>[4x]MPPMLSGLLARLVKLLLGRHGSALHWRAAGAATVLLVIVLLAGSYLACLAERGAPGAQLITYPRALWWSVETATTVGYGDLYPVTLWGRL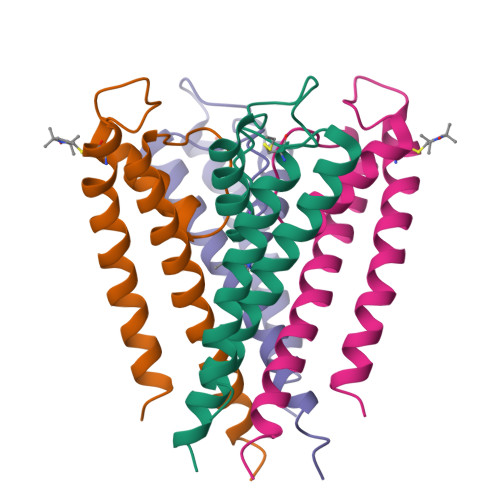VAVVVMVAGITSFGLVTAALATWFVGREQERRGHHHHHH4,4'-DIHYDROXYBIPHENYL | C12 H10 O2 | 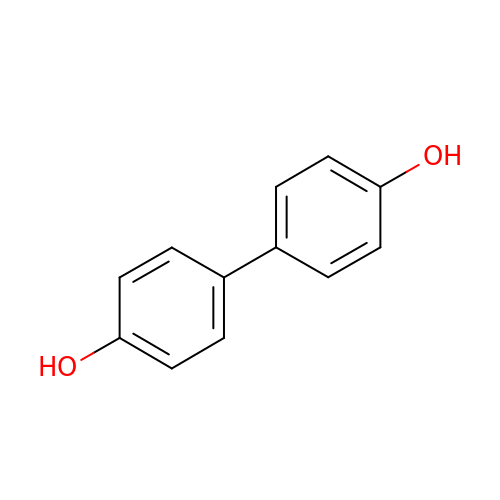VCCBEIPGXKNHFW-UHFFFAOYSA-N>[4x]HHHHHHSSGLVPRGSHMPTPSQHKDASTAQTDNQVPTGRRAQKREQTRARLITSARTLMAERGVDNVGIAEITE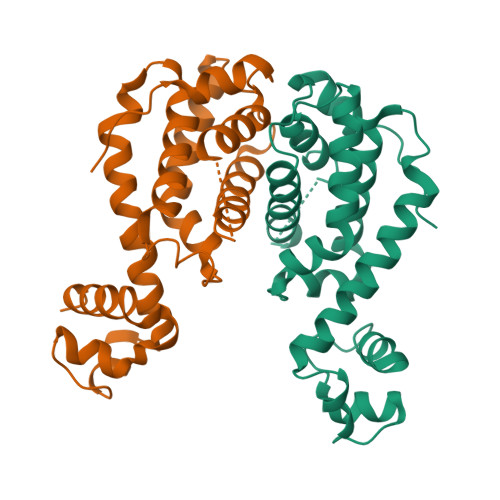GANIGTGTFYNYFPDREQLLQAVAEDAFESVGIALDQVLTKLDDPAEVFAGSLRHLVRHSLEDRIWGGFFIQMGAAHPVLMRILGPRARRDLLHGLETGRFTIEDLDLATTCTFGSLIAAIQMALSADQDSNDDKDQIFAAAMLRMVGVQAAEAREIASRPLPEISPVKPQ>[3x]MKKSLIALTLAALPVAAMADVTLYGTIKAGVETSRSVAHHGAQADRVKTATEIADLGSKIGFKGQEDLGNGLKAIWQLEQKAYVSGTDTGWGNRQSFIGLKGGFGKVRVGRLNNILKDTGNFN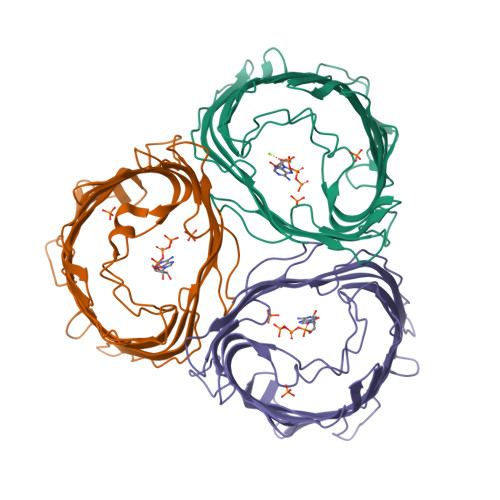PWEGKSYYSGLSNIAQPEERHVSVRYDSPEFAGFSGSVQYVPNDNSGKNRSESYHAGFNYKNDGFFVQYAGSYKRHNYTTEKHQVHRLVGGYDHDALYASVAVQQQDAKLTWRDDNSHNSQTEVATTVAYRFGNVTPRVSYAHGFKGSVYDADHDNTYDQVVVGAEYDFSKRTSALVSAGWLQKGKGAEKFVATVGGVGLRHKF;>AAAAAAAA[3x]>MSEGRRGLGRGLSALLGEVDAAPAQAPGEQLGGSREAPIEILQRNPDQPRRTFREEDLEDLSNSIREKGVLQPILVRPSPDTAGEYQIVAGERRWRAAQRAGLKTVPIMVRELDDLAVLEIGIIENVQRADLNVLEEALSYKVLMEKFERTQ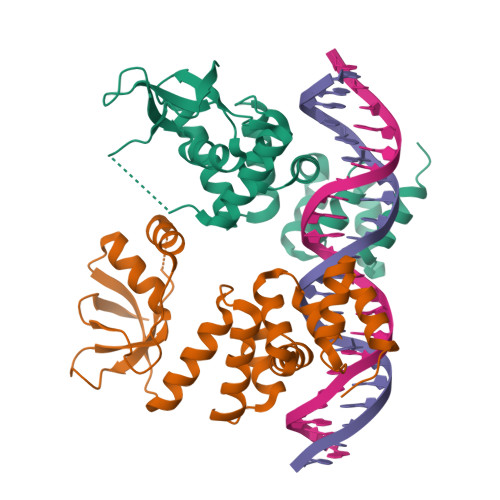ENIAQTIGKSRSHVANTMRLLALPDEVQSYLVSGELTAGHARAIAAAADPVALAKQIIEGGLSVRETEALARKAPNLSAGKSKGGRPPRVKDKLAAALEHHHHHH[4x]AFLATOXIN 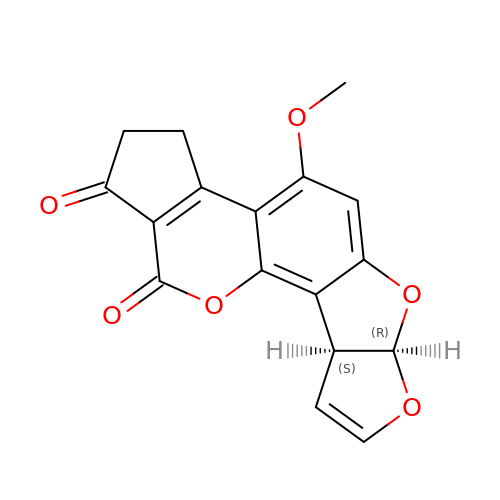B1 | C17 H12 O6 | OQIQSTLJSLGHID-WNWIJWBNSA-N The bacterial Tight adherence Secretion System (TadSS) assembles surface pili that drive cell adherence, biofilm formation and bacterial predation. Here we use cryogenic electron microscopy (cryo-EM) to reveal the architecture of the RcpA secretin in complex with TadD from P. aeruginosa. In summary, our study provides a molecular mechanism for how the TadSS secretin RcpA assembles and is coupled by its pilotin TadD to the outer membrane.

Data collection and subsequent processing steps showed that most particles fitted a C13 symmetry model whilst a subset (~5%) exhibited C14 symmetry. Working with the C13 symmetry bin, a map at 2.7 Å overall resolution was obtained. Map quality was sufficient to build a structure for the RcpA secretin between amino acids 131–383 excluding disordered residues between the tip of Gate 1 amino acids 242–255 and the S-domain between amino acids 381–416. A focussed refinement using a mask that enveloped three RcpA subunits and three TadD subunits yielded a TadD map (termed TadDFRmap) at ~4 Å resolution which enabled a TadD structure to be built between amino acids 29–212. The resulting RcpAstrep-TadDFLAG complex structure was 188 Å in diameter with RcpA forming a classical secretin-like channel decorated by TadD subunits around the outside face. The RcpA channel was partially occluded by a central gate with a 31 Å diameter opening formed between the tips of Gate 2. Above the central gate, the inner lip constricted the channel yielding a 62 Å diameter lumen. TadD packs around the secretin periphery with neighbouring subunits forming a circular filament where helix H2 in one subunit is positioned against helix H8 and the loop connecting helices H6 and H7 in the neighbouring subunit. TadD helices H3, H5, H7, H9 and H11 form the central groove and interface with RcpAaa412–416. Conserved TadD residue R79 is oriented towards and stabilises RcpA terminal residue D416, whilst TadD D139 is positioned stabilising the main chain peptide N-H group of RcpA S415.

>[13x]MHRSTGIGVSRWLGGLLGVALALPALALPQGCIELLAQAPRVDVVQGQQRDLRLAVPIERLAIGDPKIADVQLLDRRGFLVTGKEQGSTSLLIWTGCSPEPLRSLVEVEGRGSVDTRGAPAFTVGAAEELPNQVQTDIRFVEVSRSKLKQASTSFVRRGGNLWVLGAPGSLGDIKVNADGSGLGGTFGTGSSGFNLIFGGGKWLSFMNALEGSGFAYTLARPSLVAMSGQSASFLAGGEFPIPVPNGTNDNVTIEYKEFGIRLTLTPTVMNNRRIALKVAPEVSELDYSAGIQSGGVAVPALRVRRTDTSVMLADGESFVISGLTSSNSVSNVDKFPWLGDIPILGAFFRSTKLDKDDRELLMIVTPHLVQPLAADAQLPDLPGEGLRHYDPGFSRLYFLERGEYDGQQNDTGLSDSAWSHPQFEK;>MKALIGIGLCAALLGGCAALPGRDGPRECSQQLGQEQELQMNMVRDMIREGRLHAALANLESMPPGLLDVREERALILRRIGDPRARAEYQALLETCKAPEAHHGLGLLALRNGDSARAVLELREAARLRPTESRFRNDLGVALLKRGDRVGARFEFITALELQQGGKLPATNLLGLLYLQGDREDAQRLIERLQLDARDIRAAEARARSWGAVPTPGAAPASDDPLAELPAEANMHTAMANEAPGSDYKDDDDK[13x]> MAVPF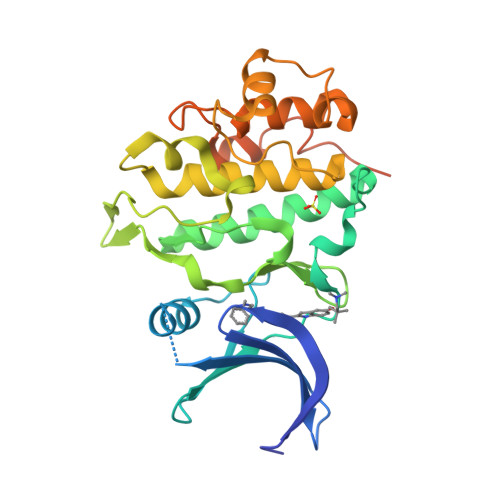VEDWDLVQTLGEGAYGEVQLAVNRVTEEAVAVKIVDMKRAVDCPENIKKEICINKMLNHENVVKFYGHRREGNIQYLFLEYCSGGELFDRIEPDIGMPEPDAQRFFHQLMAGVVYLHGIGITHRDIKPENLLLDERDNLKISDFGLATVFRYNNRERLLNKMCGTLPYVAPELLKRREFHAEPVDVWSCGIVLTAMLAGELPWDQPSDSCQEYSDWKEKKTYLNPWKKIDSAPLALLHKILVENPSARITIPDIKKDRWYNKPLKKGAKRPRVTSGGVSESPSGHHHHHHHH> MRGSHHHHHHGLVPRGSMQNPRTVSDTKRAFYAAHTRPIHSIYRRFIEELLVEIHLLRVNVDFRYSPLFALGVVTAFDQFMEGYQPEGDRDRIFHALCVAEEMNPQQLKEDAASWQQYQGRPLSQILDELNSGQPSAPLNSLNHTGKYSRLHAVGLYAFLQELAGEVTIHLNETLDQLAPVIPLPIEKVKRDLELYRSNLDKINQARSLMKELVEQERKRRAQQTSAPPAVDASSDAPA

Here we show that Psb29 in Synechocystis 6803, like THF1 in Arabidopsis, is important for normal accumulation of the FtsH heterocomplex involved in PSII repair. To gain further insights into Psb29, we have determined the crystal structure of Psb29 encoded by Thermosynechococcus elongatus, a thermophilic cyanobacterium widely used to study structural aspects of PSII assembly and repair. Each Psb29 subunit consists of 9 alpha helices. A search using PDBeFOLD found no known structures with greater than 70% similarity, indicating that the specific fold is novel.

Four crystal forms were obtained by hanging drop vapour diffusion; X-ray diffraction data were collected at resolutions from 3.6 Å to 1.4 Å and the structure of Psb29 determined by heavy atom SAD. If protease inhibitor was omitted, crystals were readily obtained in three crystal forms. Two of these were in P21 (designated A-P21 and B-P21) and the third in I222. The structure was solved by single-wavelength anomalous dispersion (SAD) with the A-P21 crystal form, soaked overnight with 1 mM dipotassium tetraiodomercurate (Jena Bioscience). Heavy atom sites for A-P21 were found and the structure phased using the autoSHARP pipeline. The initial model was built with Buccaneer and refined with REFMAC. Psb29 in the other crystal forms was proteolytically cleaved at the C-terminus. In the B-P21 crystal form, the new carboxy terminus at residue Ala189 is clearly visible in the electron density. It is likely that proteolytic cleavage of the C-terminal helix allows more compact higher resolution crystal lattices to form, as there is insufficient space in these lattices to accommodate the C-terminal helix observed in the P6322 crystal form.> MMSKVKTRIYFCGGAGFRIGELFHGYHEDVCYIDTSVQNKHKHNTDDNTIIIEADTKLADQTARKRAIGMGKDRKAAAELISAHIPAIAHHFPAGDTNIVVYSMGGASGSTIGPSLVSHLQQQGEVVVSVVIGSYDSDISLRNSSGSLKTFEGVSSVSKVPMIINYHENVEGIPQSMVNQNILEVLNALVILFNQEHQSLDLMDITNWAHFHKHHDVPVQTVQLHVCFDRQEAQAILDPIS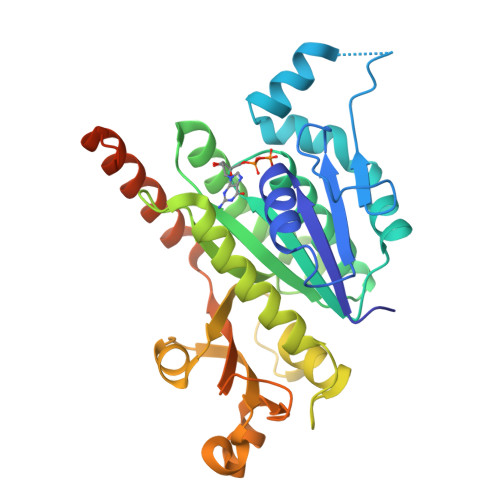IASLYTDPDRDVSISTVLTRTTGYADPEKYDFDQMHFVINGLSIEDIRKRLEERREMMNRAKANMRKRQSTLDVDDQATSSGLVFDHHHHHH> MSSEDYGYDYDLLFKIVLIGDSGVGKSNLL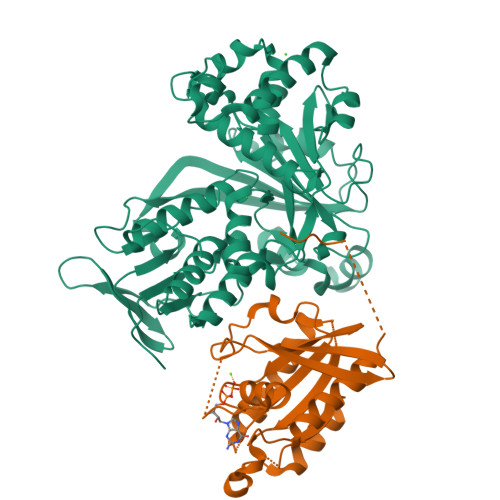SRFTKNEFNMDSKSTIGVEFATRTLEIEGKRIKAQIWDTAGQERYRAITSAYYRGAVGALIVYDISKSSSYENCNHWLSELRENADDNVAVGLIGNKSDLAHLRAVPTEESKTFAQENQLLFTETSALNSENVDKAFEELINTIYQKVSKHQMDLGDSSANGNANGASAPNGPTISLTPTPNENKKANGNNCC;> MDQETIDTDYDVIVLGTGITECILSGLLSVDGKKVLHIDKQDHYGGEAASVTLSQLYEKFKQNPISKEERESKFGKDRDWNVDLIPKFLMANGELTNILIHTDVTRYVDFKQVSGSYVFKQGKIYKVPANEIEAISSPLMGIFEKRRMKKFLEWISSYKEDDLSTHQGLDLDKNTMDEVYYKFGLGNSTKEFIGHAMALWTNDDYLQQPARPSFERILLYCQSVARYGKSPYLYPMYGLGELPQGFARLSAIYGGTYMLDTPIDEVLYKKDTGKFEGVKTKLGTFKAPLVIADPTYFPEKCKSTGQRVIRAICILNHPVPNTSNADSLQIIIPQSQLGRKSDIYVAIVSDAHNVCSKGHYLAIISTIIETDKPHIELEPAFKLLGPIEEKFMGIAELFEPREDGSKDNIYLSRSYDASSHFESMTDDVKDIYFRVTGHPLVLKQRQEQEKQ>[4x]QGLLAGK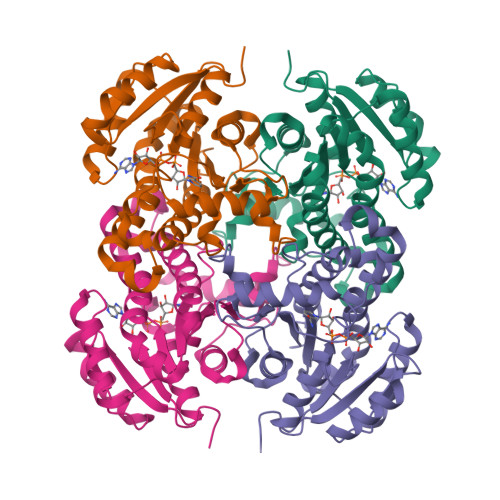RFLIAGVASKLSIAYGIAQALHREGAELAFTYPNEKLKKRVDEFAEQFGSKLVFPCDVAVDAEIDNAFAELAKHWDGVDGVVHSIGFAPAHTLDGDFTDVTDRDGFKIAHDISAYSFVAMARAAKPLLQARQGCLLTLTYQGSERVMPNYNVMGMAKASLEAGVRYLASSLGVDGIRVNAISAGPIRTLAASGIKSFRKMLDANEKVAPLKRNVTIEEVGNAALFLCSPWASGITGEILYVDAGFNTVGMSQS> MSGSMEGNAVSFKGGVFSPYLTTRLPAWAGVRQNVMGSNVDGRPVAPANSATLTYATVGSSVDTAAAAAASAAASTARGMAADFGLYNQLAASRSLREEDALSVVL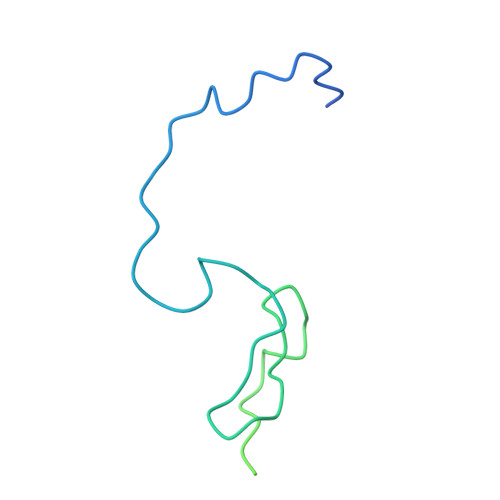TRLEELSQQLQDLFAKVALLNPPANAS> AGYPPASPSNLSCLMHLTTNSLVCQWEPGPETHLPTSFILKSFRSRADCQYQGDTIPDCVAKKRQNNCSIPRKNLLLYQYMAIWVQAENMLGSSESPKLCLDPMDVVKLEPPMLQALDIGPDVV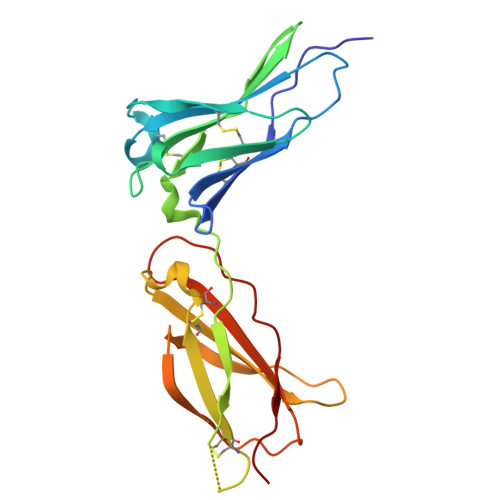SHQPGCLWLSWKPWKPSEYMEQECELRYQPQLKGANWTLVFHLPSSKDQFELCGLHQAPVYTLQMRCIRSSLPGFWSPWSPGLQLRPTMKA> PKALIVYGSTTGNTEYTAETIARELADAGYEVDSRDAASVEAGGLFEGFDLVLLGCSTWLDDSIELQDDFIP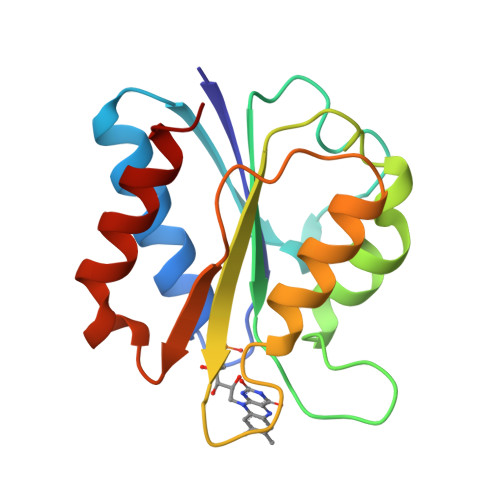LFDSLEETGAQGRKVACFGCGDSSYEYFCGAVDAIEEKLKNLGAEIVQDGLRIDGDPRAARDDIVGWAHDVRGAI6-[4-(aminomethyl)-2-fluorophenoxy]-2,1-benzoxaborol-1(3H)-ol | C14 H13 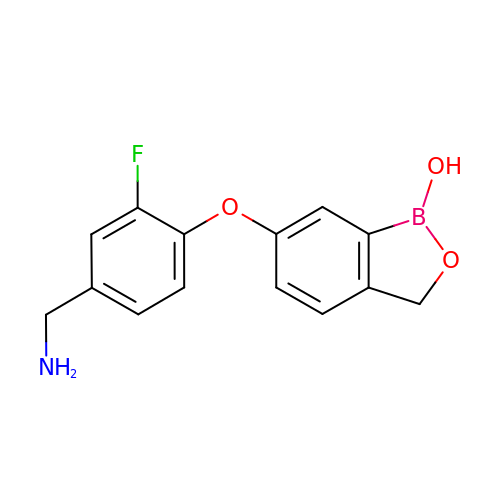B F N O3 | TUWUQFIFQVYZSK-UHFFFAOYSA-N>MAPTFQTALFFTIISLSFAAPNAKQVRWCAISDLEQKKCNDLVGSCNVPDITLVCVLRSSTEDCMTAIKDGQADAMFLDSGEVYEASKDPYNLKPIIAEPYSSNRDLQKCLKERQQALAKKMIGHYIPQCDEKGNYQPQQCHGSTGHCWCVNAMGEKISGTNTPPGQTRATCERHELPKCLKERQVALGGDEKVLGRFVPQCDEKGNYEPQQFHGSTGYSWCVNAIGEEIAGTKTPPGKIPATCQKHDLVTTCHYAVAMVKKSSAFQFNQLKGKRSCHSGVSKTDGWKALVTVLVEKKLLSWDGPAKESIQRAMSKFFSVSCIPGATQTNLCKQCKGEEGKNCKNSHDEPYYGNYGAFRCLKEDMGDVAFLRSTALSDEHSEVYELLCPDNTRKPLNKYKECNLGTVPAGTVVTRKISDKTEDINNFLMEAQKRQCKLFSSAHGKDLMFDDSTLQLALLSSEVDAFLYLGVKLFHAMKALTGDAHLPSKNKVRWCTINKLEKMKCDDWSAVSGGAIACTEASCPKGCVKQILKGEADAVKLEVQYMYEALMCGLLPAVEEYHNKDDFGPCKTPGSPATDFGTLRAVALVKKSNKDINWNNIKGKKSCHTGVGDIAGWVIPVSLIRRQNDNSDIDSFFGESCAPGSDTKSNLCKLCIGDPKNSAANTKCSLSDKEAYYGNQGAFRCLVEKGDVAFVPHTVVFENTDGKNPAVWAKNLKSEDFELLCLDGSRAPVSNYKSCKLSGIPPPAIVTREESISDVVRIVANQQSLYGRKGFEKDMFQLFSSNKGNNLLFNDNTQCLITFDRQPKDIMEDYFGKPYYTTVYGASRSA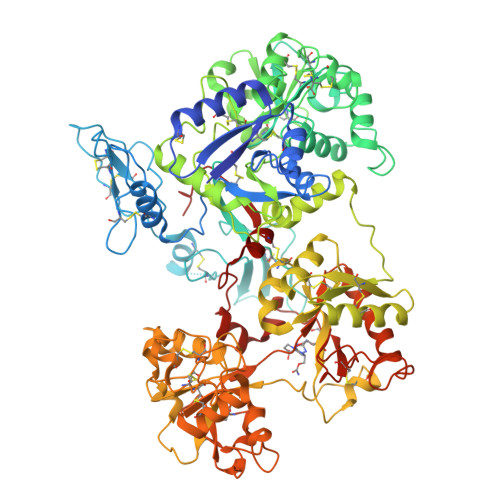MSSELISACTIKHCSNSLEVL[2x]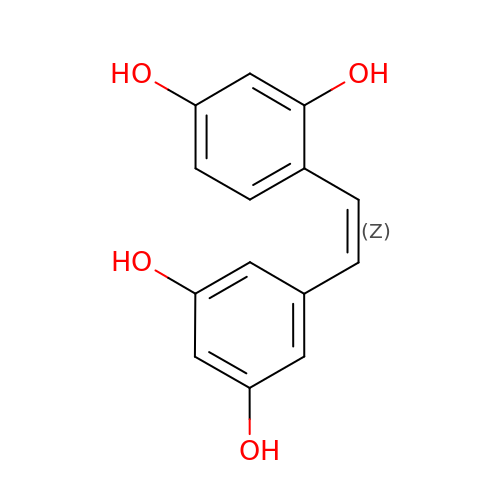cis-oxyresveratrol | C14 H12 O4 | PDHAOJSHSJQANO-UPHRSURJSA-N>[4x]MATKTSIHPSVNELYQRLAEDQLSNCFDRFDPQEKIRCNYCELGVSCQLCSNGPCRINEKVGATLGVCGINADGMAMRYMLLRNVMGTSTYTYHAYEAYKTLKMTALGNTPFTITDKDKLYQMAKDLELNTEGKPEDVAVRLSD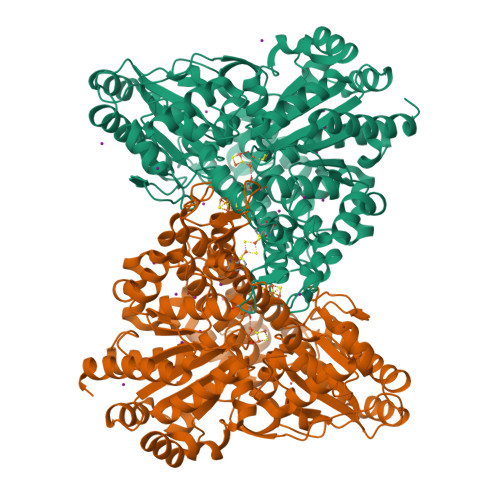FLIWELYRDYDEPGKMIEVYAPLKRKEVWRKLGIYPAGPLHELKDAAASCLTNVDGDYVSLATKGLRLGLSCIYGAQIGLELVQDILFGTGMPHEMDVDLGIFDADYINIVFNGHEPFVGVALILAAKEAVNQDKAKAAGAKSLRIYGSIESGQEVVQRFQKDEVFRGLTGNWLTIEPMLATGAVDVLAMDMNCSPPNLGPLAEKYGATLVSVSRLVRFPGIHHFLDYKPSEVREIAQKIIDIAVDSFKNKRHGKITPKIPANIQKAITGFTPEAILKALGGSINPLIEVIKAGKIKGAVGLINCTTLKNGPQDYVTVNLAKELIKRDILILSGGCGNHALEVAGLCNLDAINLAGPGLSEVCRNLNIPPVLSFGTCTDTGRISLVVTALANALNVDTADLPVAVTAPMYMEQKATIDALFALAYGLYTHVAPDPPVMGAPNLVKLLTRDLPSITGGRIAVGSDPVKVADDILAHINDRRAKLGI> GSAKDPSRKSNVTGDALSASVGVGVPIQDIKVDVQNLAQGDINELGAKFSSRDDIFSQVDTTLKFYTQNKDYAVNIKAGMTLGDVAQSITDATNGEVMGIVMKTGGNDPYQLMVNTKNTGEDNRVYFGSHLQSTLTNKNALSLGVDGSGKSEVSLNLKGADGNMHEVPIMLELPESASIKQKNTAIQKAMEQALENDPNFKNLIANGDISIDTLHGGESLIINDRRGGNIEVKGSKAKELGFLQTTTQESDLLKSSRTIKEGKLEGVVSLNGQKLDLSALTKESNTSEE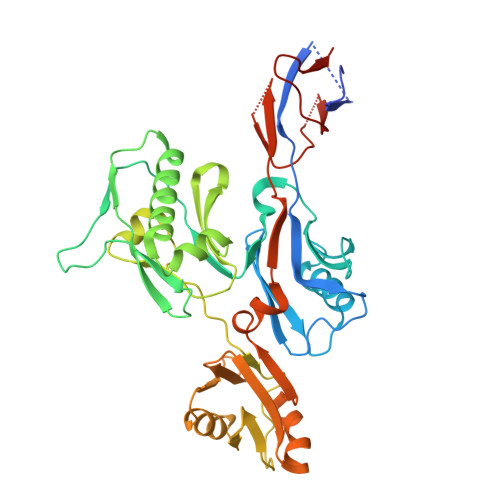NTDAIIQAINAKEGLSAFKNAEGKLVINSKTGMLTIKGEDALGKASLKDLGLNAGMVQSYEASQNTLFMSKNLQKASDSAFTYNGVSITRPTNEVNDVISGVNITLEQTTEPNKPAIISVSRD> MKLKKIVFTLIALGLFSCKTTSVLVKNEPQLKTPKNVILLISDGAGLSQISSTFYFKEGTPNYTQFKNIGLIKTSSSREDVTDSASGATAFSCGIKTYNAAIGVADDSTAVKSIVEIAALN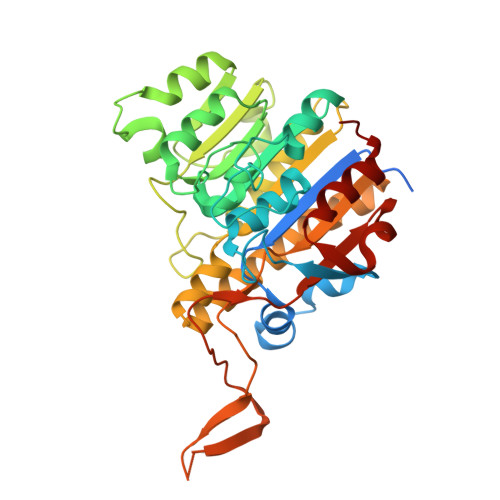NIKTGVVATSSITHATPASFYAHALNRGLEEEIAMDMTESDLDFFAGGGLNYFTSRKDKKDVLAILKGNQFTINTTGLTDFSSIASNRKMGFLLADEAMPTMESGRGNFLSAATDLAIQFLSKDNSAFFIMSEGSQIDWGGHANNASYLISEINDFDDAIGTALAFAKKDGNTLVIVTSDHETGGFTLAAKKNKREDGSEYSDYTSIGPSFSTGGHSATLIPVFAYGPGSEEFIGIYENNEIFHKILKVTKWNQ> SQN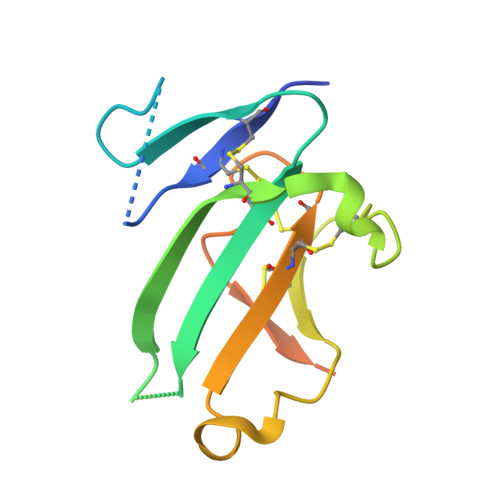QERLCAFKDPYQQDLGIGESRISHENGTILCSKGSTCYGLWEKSKGDINLVKQGCWSHIGDPQECHYEECVVTTTPPSIQNGTYRFCCCSTDLCNVNFTENFPPPDTTPLSPPHSFNRDET> MGEEDYYLELCERPVQFEKANPVNCVFFDEANKQVFAVRSGGATGVVVKGPDDRNPISFRMDDKGEVKCIKFSLENKILAVQRTSKTVDFCNFIPDNSQLEYTQECKTKNANILGFCWTSSTEIVFITDQGIEFYQVLPEKRSLKLLKSHNLNVNWYMYCPESAVILLSTTVLENVLQPFHFRAGTMSKLPKF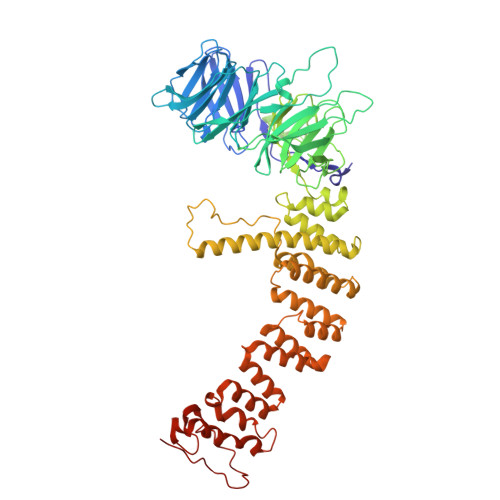EIELPAAPKSTKPSLSERDIAMATIYGQLYVLFLRHHSRTSNSTGAEVVLYHLPREGACKKMHILKLNRTGKFALNVVDNLVVVHHQDTETSVIFDIKLRGEFDGSVTFHHPVLPARSIQPYQIPITGPAAVTSQSPVPCKLYSSSWIVFQPDIIISASQGYLWNLQVKLEPIVNLLPDKGRLMDFLLQRKECKMVILSVCSQMLSESDRASLPVIATVFDKLNHEYKKYLDAEQSYAMAVEAGQSRSSPLLKRPVRTQAVLDQSDVYTHVLSAFVEKKEMPHKFVIAVLMEYIRSLNQFQIAVQHYLHELVIKTLVQHNLFYMLHQFLQYHVLSDSKPLACLLLSLESFYPPAHQLSLDMLKRLSTANDEIVEVLLSKHQVLAALRFIRGIGGHDNISARKFLDAAKQTEDNMLFYTIFRFFEQRNQRLRGSPNFTPGEHCEEHVAFFKQIFGDQALMRPTTF>[4x]MANVNKTPGKTRRAEVAGGGFAGLTAAIALKQNGWDVRLHEKSSELRAFGAGIYLWHNGLRVLEGLGALDDVLQGSHTPPTYETWMHNKSVSKETFNGLPWRIMTRSHLHDALV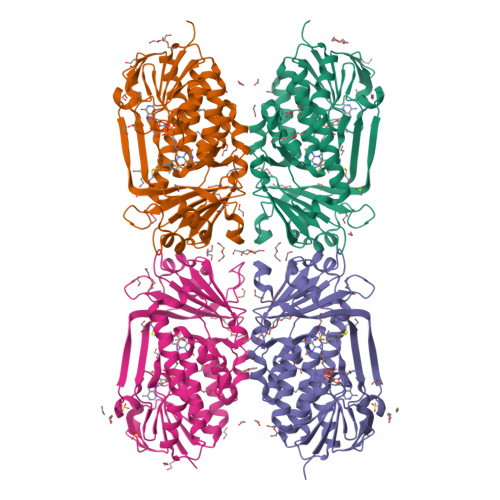NRARALGVDISVNSEAVAADPVGRLTLQTGEVLEADLIVGADGVGSKVRDSIGFKQDRWVSKDGLIRLIVPRMKKELGHGEWDNTIDMWNFWPRVQRILYSPCNENELYLGLMAPAADPRGSSVPIDLEVWVEMFPFLEPCLIEAAKLKTARYDKYETTKLDSWTRGKVALVGDAAHAMCPALAQGAGCAMVNAFSLSQDLEEGSSVEDALVAWETRIRPITDRCQALSGDYAANRSLSKGNMFTPAALEAARYDPLRRVYSWPQ> MSSEDY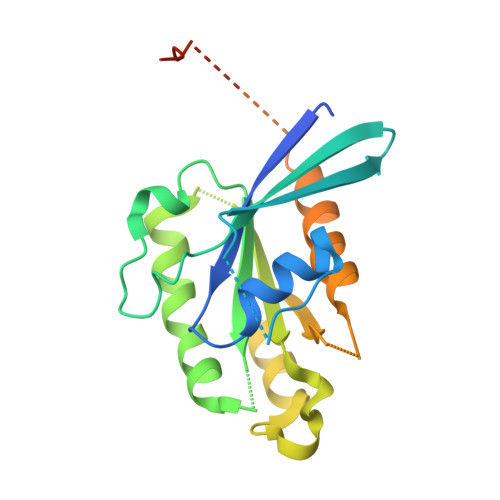GYDYDLLFKIVLIGDSGVGKSNLLSRFTKNEFNMDSKSTIGVEFATRTLEIEGKRIKAQIWDTAGQERYRAITSAYYRGAVGALIVYDISKSSSYENCNHWLSELRENADDNVAVGLIGNKSDLAHLRAVPTEESKTFAQENQLLFTETSALNSENVDKAFEELINTIYQKVSKHQMDLGDSSANGNANGASAPNGPTISLTPTPNENKKANGNNCC3-chloranyl-~{N}-[(1~{S})-1-(6-chloranylpyridin-3-yl)-2-phenyl-ethyl]aniline | C19 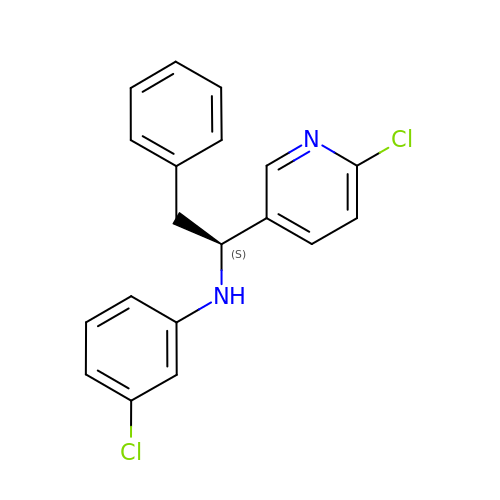H16 Cl2 N2 | FPQMXEJXTNDYME-SFHVURJKSA-N>[2x]MENTENSVDSKSIKNLEPKIIHGSESMDSGISLDNSYKMDYPEMGLCIIINNKNWHKSTGMTSRSGTDVDAANLRETFRNLKYEVRNKNDLTREEIVELMRDVSKEDHSKRSSFVCVLLSHGEEGIIFGTNGPVDLKKITNFFRGDRCRSLTGKPKLFIIQACRGTELDCGIETDSG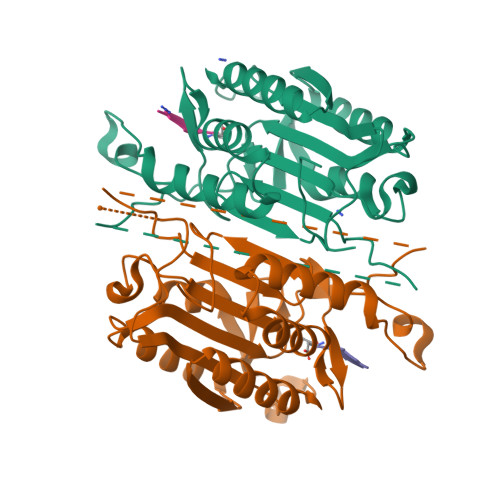VDDDMACHKIPVEADFLYAYSTAPGYYSWRNSKDGSWFIQSLCAMLKQYADKLEFMHILTRVNRKVATEFESFSFDATFHAKKQIPCIVSMLTKELYFYHL3-[(2~{S},3~{R},4~{R})-4-[[(2~{S})-2-azanyl-3-methyl-butanoyl]amino]-2-carboxy-pyrrolidin-3-yl]propyl-$l^{3}-oxidanyl-bis(oxidanyl)boron 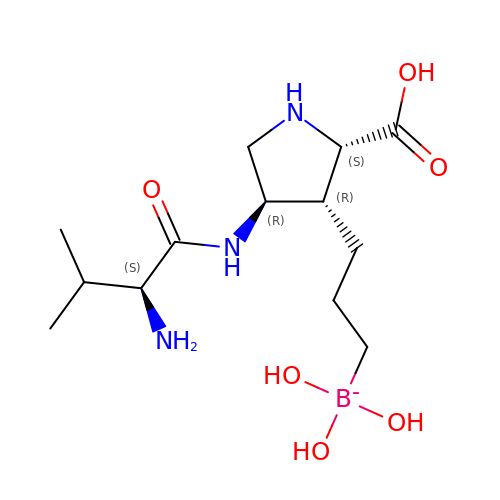| C13 H27 B N3 O6 | BIHQJUDSCKNIPN-RCWTZXSCSA-N>THPDISVDVLVIGAGPTGLGAAKRLNQIDGPSWMIVDSNETPGGLASTDVTPEGFLYDVGGHVIFSHYKYFDDCLDEALPKEDDWYTHQRISYVRCQGQWVPYPFQNNISMLPKEEQVKCIDGMIDAALEARVANTKPKTFDEWIVRMMGTGIADLFMRPYNFKVWAVPTTKMQCAWLGEKVAAPNLKAVTTNVILGKTAGNWGPNATFRFPARGGTGGIWIAVANTLPKEKTRFGEKGKVTKVNANNKTVTLQDGTTIGYKKLVSTMAVDFLAEAMNDQELVGLTKQLFYSSTHVIGVGVRGSRPERIGDKCWLYFPEDNCPFYRATIFSNYSPYNQPEASKKLPTMQLADGSRPQSTEAKEGPYWSIMLEVSESSMKPVNQETILADCIQGLVNTEMLKPTDEIVSTYHRRFDHGYPTPTLEREGALTQILPKLQDKDIWSRGRFGSWRYEVGNQDHSFMLGVEAVDNI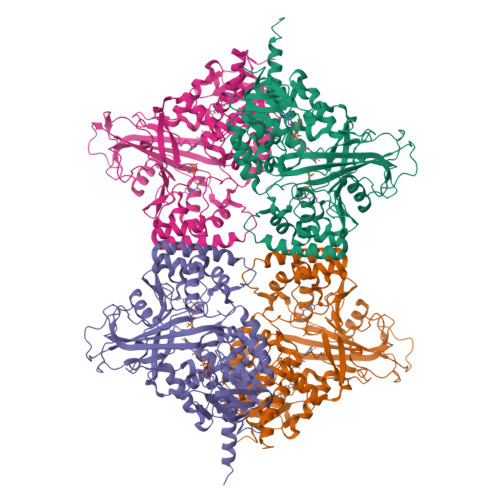VNGAVELTLNYPDFVNGRQNTERRLVDGAQVFAKSKAQLEHHHHHH[4x]>[4x]MAPIEWESSPRVEVFVGRKRELSIIRNAKGVVVIYGIAGIGKTSLAAKAFPNAYWYNVTGLEDFKYFAWQLGLFLSSIGFEDLLEYLRGGGNNENDIFKLITEGIEKTGAIIIIDDFHKFQDEKVNYLLSYLAPRIKKGKVIITTRIRPNLGNEGVTYVNLKGLNPEEAYSLAREKEKSMTPEEFAKLYKLTFGHPLMLNLILESSEILATGKDTVFNFLFEEVYQMLNEEEKDLLSILSLFDEPIEYEGIKFLYDRNPFVPLYSLMKKGLIEKKGEKYFVHDMVREFVREVSNQEEKEVYLRHVNFLLKSKTPINFLRAFKYAIKVGSSELIRNLVELRVKEFYRIIVDFPRMYQRLLMEVEDNPYAKIEIAIIEVQRGLFEKAIKLLKEAEPYVDEFFKCEIYSWLADAYMELENLEKAERYLKKTKEIVEKINDMYAWFSYYAEKTKYEYYKENSREALKSALKELEIIRKIGDPEKEGLVLLHVGDIYLHMGNYEKGISYYQEALKMAKAYGIKFLEHISYMELAKGYYQLKLYEKASEYSEKAANYFLMIRNYRRATDAMAYGSVSYIATKNLEKAEKFAKEMIRIAQSTDYPLAWAGYIFLAAVDFLKGDDWREDYNLGKAHLKEYPWLFEAVLDELKKVFDLSNFK

Signal transduction ATPases with numerous domains (STAND) are a family of AAA+ related ATPases involved in a wide range of cellular activities. The hallmark of STAND ATPases is a conserved core called nucleotide-binding oligomerization domain (NOD), which is responsible for nucleotide binding and protein oligomerization. In most cases, the NOD is followed by an arm domain and a non-conserved sensor domain made of repeated motifs, which was found to contain the primary inducer-binding site in several instances. PH0952 is a predicted transcription factor with a TPR sensor domain and a putative N-terminal ArsR-like DNA-binding effector domain.

Native crystals of PH0952 lacking its N-terminal effector domain belonged to space group P65 and diffracted X-rays to 3.4 Å. The asymmetric unit contained four protein molecules with RMSD values lower than 0.38 Å among 641 αC atoms. Each PH0952ΔN molecule exhibits a curled up conformation in the shape of the letter G, with 90 × 60 × 40 Å3 dimensions. In the putative nucleotide-binding site, a ligand was clearly visible in the experimental electron density map and was interpreted as an ADP molecule (present in the buffer). The domain organization of the protein is that of a bona fide STAND protein in the monomeric resting state, consistent with the presence of a diphosphate nucleotide. It comprises a NOD module with three domains: the three-layered α/β nucleotide-binding domain (NBD, amino acids 102–262), the helical domain (HD, amino -acids 263–316) and the winged-helix domain (WHD, amino acids 317–393). The NOD is followed by an arm domain (also named HD2, amino acids 394–496) and a sensor domain (amino -acids 497–748) composed of tetratricopeptide repeats. The buried surface area between the arm and the NBD of PH0952 is 490 Å2, consistent with the key role of the arm in the STAND autoinhibition process. Finally, the PH0952 TPR sensor caps the tip of the NBD that is formed by helices ISM (α3), ISMb (α4) and H2 (α5), burying a surface of 360 Å, similar to the NBD–WHD and NBD–arm interfaces. Thus, the NBD is clamped between the arm and the sensor domain, suggesting that in the crystal, PH0952 is autoinhibited by NBD–arm and NBD–sensor interactions.> GSSTVTLPETLLFVSTLDGSLHAVSKRTGSIKWTLKEDPVLQVPTHVEEPAFLPDPNDGSLYTLGSKNNEGLTKLPFTIPELVQASPCRSSDGILYMGKKQDIWYVIDLLTGEKQQTLSSAFADSLSPSTSLLYLGRTEYTITMYDTKTRELRWNATYFDYAASLPEDDVDYKMSHFVSNGDGLVVTVDSESGDVLWIQNYASPVVAFYVWQREGLRKVMHINVAVETLRYLTFMSGEVGRITKWKYPFPKETEAKSKLTPTLYVGKYSTSLYASPSMVHEGVAVVPRGSTLPLLEGPQTDGVTIGDKGESVITPSTDVKFDPGLKSKNKLNYLR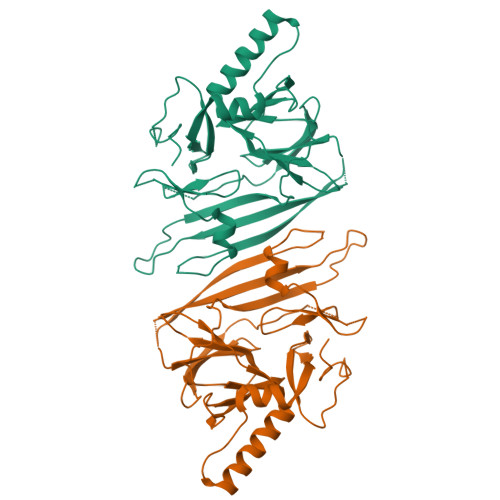NYWLLIGHHETPLSASTKMLERFPNNLPKHRENV> GYVPAVVIGTGYGAAVSALRLGEAGVQTLMLEMGQLWNQPGPDGNIFCGMLNPDKRSSWFKNRTEAPLGSFLWLDVVNRNIDPYAGVLDRVNYDQMSVYVGRGVGGGSLVNGGMAVEPKRSYFEEILPRVDSSEMYDRYFPRANSMLRVNHIDTKWFEDTEWYKFARVSREQAGKAGLGTVFVPNVYDFGYMQREAAGEVPKSALATEVIYGNNHGKQSLDKTYLAAALGTGKVTIQTLHQVKTIRQTKDGGYALTVEQKDTDGKLLATKEISCRYLFLGAGSLGSTELLVRARDTGTLPNLNSEVGAGWGPNGNIMTARANHMWNPTGAHQSSIPALGIDAWDNSDSSVFAEIAPMPAGLETWVSLYLAITKNPQRGTFVYDAATDRAKLNWTRDQNAPAVNAAKALFDRINKANGTIYRYDLFGTQLKAFADDFCYHPLGG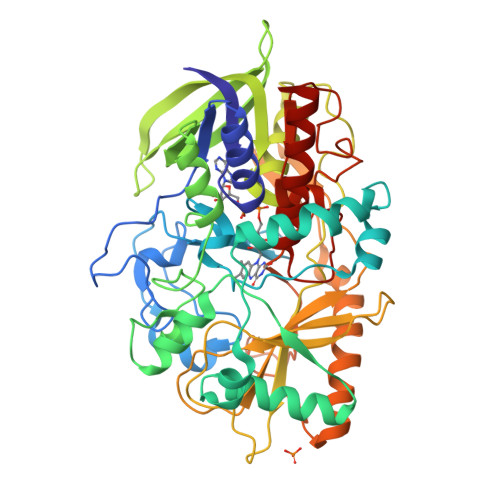CVLGKATDDYGRVAGYKNLYVTDGSLIPGSVGVNPFVTITALAERNVERIIKQDVT>[2x]GSHMGRKFFVGGNWKCNG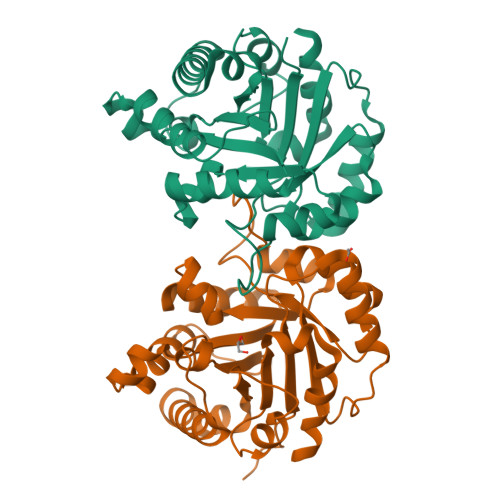TTDQVEKIVKTLNEGQVPPSDVVEVVVSPPYVFLPVVKSQLRQEFHVAAQNCWVKKGGAFTGEVSAEMLVNLGVPWVILGHSERRALLGESNEFVGDKVAYALSQGLKVIACVGETLEQREAGSTMDVVAAQTKAIAEKIKDWSNVVVAYEPVWAIGTGKVATPAQAQEVHASLRDWLKTNASPEVAESTRIIYGGSVTAANCKELAAQPDVDGFLVGGASLKPEFIDIINAATVKSA>MTNSNHKNLTTNQGVPVGDNQNSRTAGHRGPSFLDDYHLIEKLAHFDRERIPERVVHARGAGAYGVFEVENSMEKHTRAAFLSEEGKQTDVFVRFSTVIHPKGSPETLRDPRGFAVKFYTEEGNYDLVGNNLPIFFIRDALKFPDMVHSLKPDPVTNIQDPDRYWDFMTLTPESTHMLTWLFSDEGIPANYAEMRGSGVHTFRWVNKYGETKYVKYHWRPSEGIRNLSMEEAAEIQANDFQHATRDLYDRIEKGNYPAWDLYVQLMPLSDYDELDYDPCDPTKTWSEEDYPLQKVGRMTLNRNPENFFAETEQAAFTPSALVPGIEASEDKLLQGRLFSYPDTQRHRLGANYMRIPVNCP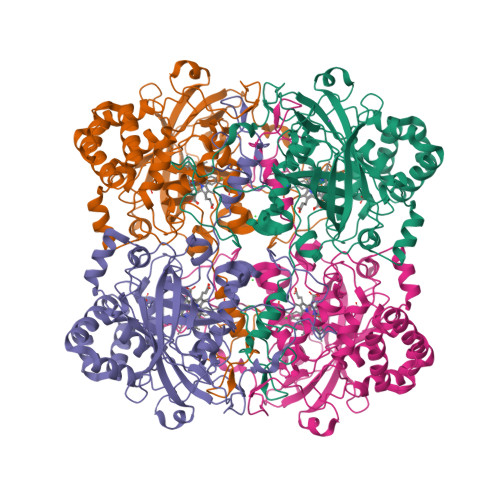YAPVHNNQQDGFMTTTRPSGHINYEPNRYDDQPKENPHYKESEPVLHGDRMVRQKIEKPNDFKQAGEKYRSYSEEEKQALIKNLTADLKGVNEKTKLLAICNFYRADEDYGQRLADSLGVDIRSYLQGSMK[4x]> ASVHGTTYELLRRQGIDTVFGNPGSNELPFLKDFPEDFRYILALQEACVVGIADGYAQASRKPAFINLHSAAGTGNAMGALSNAWNSHSPLIVTAGQQTRAMIGVEALLTNVDAANLPRPLVKWSYEPASAAEVPHAMSRAIHMASMAPQGPVYLSVPYDDWDKDADPQSHHLFDRHVSSSVRLND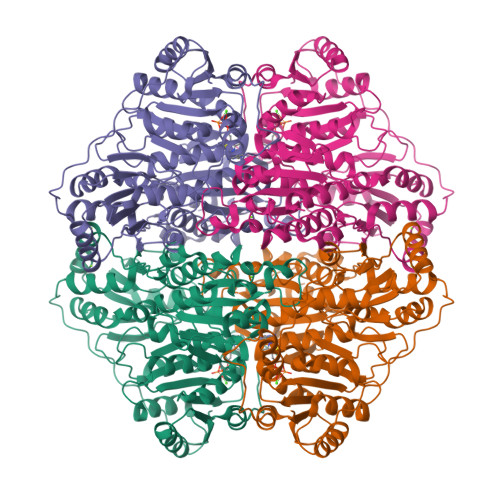QDLDILVKALNSASNPAIVLGPDVDAANANADCVMLAERLKAPVWVAPSAPRCPFPTRHPCFRGLMPAGIAAISQLLEGHDVVLVIGAPVFRYNQYDPGQYLKPGTRLISVTCDPLEAARAPMGDAIVADIGAMASALANLVEESSRQLPTAAPEPAKVDQDAGRLHPETVFDTLNDMAPENAIYLNESTSTTAQMWQRLNMRNPGSYYFCAAGGLGFALPAAIGVQLAEPERQVIAVIGDGSANYSISALWTAAQYNIPTIFVIMNNGTYGALRWFAGVLEAENVPGLDVPGIDFRALAKGYGVQALKADNLEQLKGSLQEALSAKGPVLIEVSTVSHHHHHH>[4x]MKVFNRPILFDIVSRGSPDGLEGLLSFLLTHKKRLTDEEFREPSTGKTCLPKALLNLSAGRNDTIPILLDIAEKTGNMREFINSPFRDVYYRGQTALHIAIERRCKH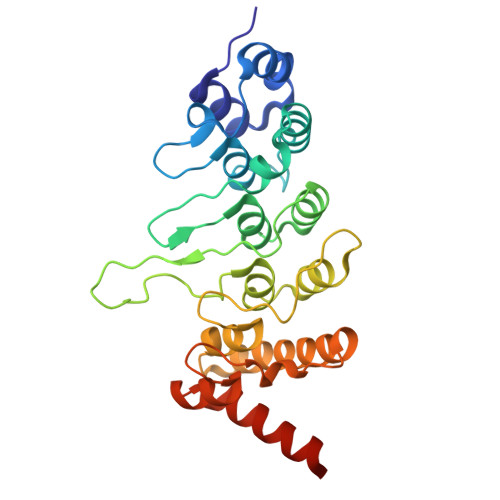YVELLVEKGADVHAQARGRFFQPKDEGGYFYFGELPLSLAACTNQPHIVHYLTENGHKQADLRRQDSRGNTVLHALVAIADNTRENTKFVTKMYDLLLIKCAKLFPDTNLEALLNNDGLSPLMMAAKTGKIGIFQHIIRREIADAAAHHHHHH>[4x]SAQVGTNKELCCLVYTSWQIPQKFIVDYSETSPQCPKPGVILLTKRGRQICADPNK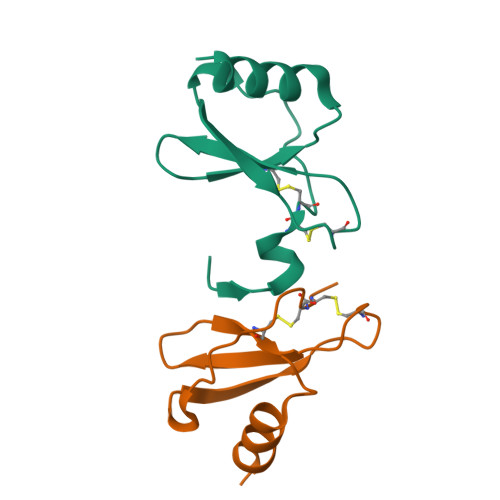KWVQKYISDLKLNA> SNAGKNVMVEPHRHEGVFICRGKEDALVTKNLVPGESVYGEKRVSISEGDDKIEYRAWNPFRSKLAAAILGGVDQIHIKPG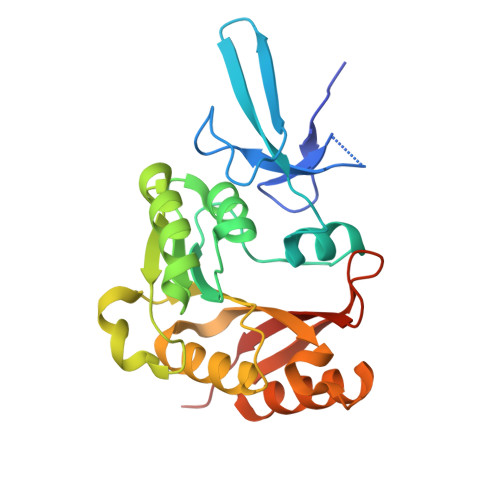AKVLYLGAASGTTVSHVSDIVGPDGLVYAVEFSHRSGRDLINLAKKRTNIIPVIEDARHPHKYRMLIAMVDVIFADVAQPDQTRIVALNAHTFLRNGGHFVISIKANCIDSTASAEAVFASEVKKMQQENMKPQEQLTLEPYERDHAVVVGVYRPPPKVKN Here, we exploit the relience of Mtb on host-derived cholesterol to develop a novel class of antitubercular compounds that target Mtb CYP125 and CYP142; the enzymes that catalyze the first step of cholesterol metabolism. The first step of cholesterol degradation in MtbC27-oxidation of the cholesterol/enone side chain―is catalyzed by a 48 kDa cytochrome p450 enzyme (P450), CYP125. − Cyp125 (Rv3545c) is encoded in the Mtb intracellular growth (igr) operon, which is widely conserved across actinomycetes and is essential for Mtb survival in macrophages and mice. (A) Mtb cholesterol metabolism: CYP125 and CYP142 catalyze C27-oxidation of cholest-4-en-3-one to yield cholestenoic acid, which is subsequently degraded to androstendione, acetyl CoA, and propionyl CoA. We subsequently employ CYP142 as a structural proxy to guide hit-to-lead optimization of dual CYP125/142 inhibitors that have low nanomolar binding affinity and inhibit CYP125/142 catalytic activity in vitro.

A combination of improvements made to CYP125 expression and crystallization conditions during the synthetic optimization of 1a, in addition to the tight binding affinity of the dual CYP125/142 inhibitors, enabled us to obtain high resolution X-ray crystal structures of compounds 5j and 5m in complex with CYP125 and CYP142 (and compound 5g in complex with CYP125). In all 4 structures, the pyridine-nitrogen of the inhibitor directly coordinated to the P450 heme iron, consistent with their type II optical spectra and the binding mode of 1a–i to CYP142. In contrast, the conformation of the sulfonamide linker in compound 5j directs the phenyl substituent away from binding pocket of 1a -ii and introduced disfavorable interactions with CYP142_Met74. This conformation might account for the weaker binding affinity of compounds that contain a sulfonamide (e.g., 3g, 5k) or amide linker (e.g., 5a–d) relative to their benzylamine analogues (e.g., 5l–p), and is consistent with the comparatively weak affinity of CYP142 to fragments containing a sulfonamide substituent, which was noted in the original SAR screen (e.g., 3g). Binding interactions between CYP142 and 5m or 5j were exclusively hydrophobic (and metal co-ordination), while CYP125 also formed key hydrogen bonding interactions with the amine/sulfonamide linker (5m/5j) and methoxy group (5m) of the ligands via Glu112 and Ser217, respectively. These additional interactions likely contribute to tighter binding affinity and improved inhibition of CYP125 verse CYP142 by 5m and 5j. In all CYP125 co-crystal structures, the pyridine ring of the inhibitor was rotated 90 degrees relative to that observed for the same inhibitor in complex with CYP142, and the orientation of the 1a–i pyridine ring in the original CYP142-1a structure.

> GTEAPDVDLADGNFYASREARAAYRWMRANQPVFRDRNGLAAASTYQAVIDAERQPELFSNAGGIRPDQPALPMMIDMDDPAHLLRRKLVNAGFTRKRVKDKEASIAALCDTLIDAVCERGECDFVRDLAAPLPMAVIGDMLGVRPEQRDMFLRWSDDLVTFLSSHVSQEDFQITMDAFAAYNDFTRATIAARRADPTDDLVSVLVSSEVDGERLSDDELVMETLLILIGGDETTRHTLSGGTEQLLRNRDQWDLLQRDPSLLPGAIEEMLRWTAPVKNMCRVLTADTEFHGTALCAGEKMMLLFESANFDEAVFCEPEKFDVQRNPNSHLAFGFGTHFCLGNQLARLELSLMTERVLRRLPDLRLVADDSVLPLRPANFVSGLESMPVVFTPSPPLG>[2x]GHMASTSSLTPPKTMFIVGSMLDTDWKVWKPMAGVYGMDGQFYSMIYFDANSEFKFGTKENEYIGINDNRVTVTDKAGAGVSGSDNFVVENAG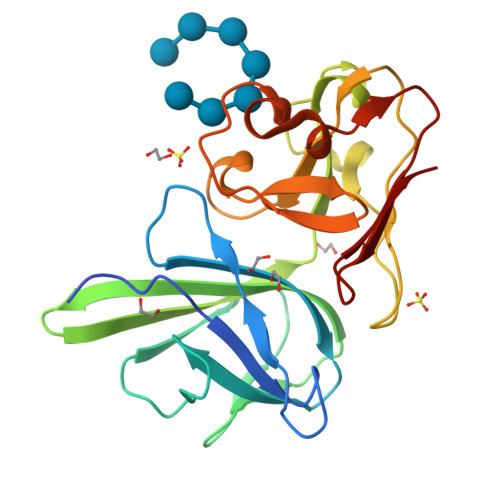WYLFYVKAAVKGDDYQFTITFYPAEVYLFGNTTGGSWAFNDEWKFTVPATKDGNFVSPAMTASGEVRMCFKTDLDWWRTEFTLHDGEIFYRDFNLIDSWTEKGDGYSIQGSAGNVIHLNFTAGTGEKK While chemical methylation of an amide bond uses a strong base to generate the imidate, OphA, the precursor protein of the fungal peptide macrocycle omphalotin A, self-hypermethylates amides at pH 7 using S-adenosyl methionine (SAM) as cofactor. Omphalotin A derives from the C terminus of the OphA protein, and it is the OphA protein that methylates its own C terminus using S-adenosyl methionine (SAM). The structure of OphA reveals a complex catenane-like arrangement in which the peptide substrate is clamped with its amide nitrogen aligned for nucleophilic attack on the methyl group of SAM. Here, we report the structure of the peptide amide methyltransferase OphA including complexes with cofactor [SAM and S-adenosyl homocysteine (SAH)], cofactor analog, substrate, and product.

Y76F and Y98A led to highly aggregated protein, and only a small amount could be purified for analysis; very little folded material was obtained for Y98F, but no methylation was detected. Y76F, R72A, R72K, and Y98A were unmethylated even after 3 days of overexpression in E. coli. A different conformation of Tyr98 is seen in inactive mutant complexes (Y76F-SAM, Y76F-SAH, and R72A-SAH). In addition, complexes R72A-SAH and Y76F-SAH show similar active conformation of the substrate peptide. We predict that removal of the methyl group of SAM by changing to SAH would remove the “driving force” for the flipped conformation. The structures of R72A and Y76F with SAH do show the active conformation.

>[2x]GTSTQTKAGSLTIVGTGIESIGQMTLQALSYIEAAAKVFYCVIDPATEAFILTKNKNCVDLYQYYDNGKSRLNTFTQMSELMVREVRKGLDVVGVFYGHPGVFVNPSHRALAIAKSEGYRARMLPGVSAEDCLFADLCIDPSNPGCLTYEASDFLIRDRPVSIHSHLVLFQVGCVGIADFNFTGFDNNKFGVLVDRLEQEYGAEHPVVHYIAAMMPHQDPVTDKYTVAQLREPEIAKRVGGVSTFYIPPKARKASNLDIIRRLELLPAGQVPDKKARIYPANQWEPDVPEVEPYRPSDQAAIAQLADHAPPEQYQPLATSKAMSDVMTKLALDPKALADYKADHRAFAQSVPDLTPQERAALELGDSWAIRCAMKNMPSSLLDAARESGEEASQNGFPWVIVVGVIGVIG>[2x]MNSKIRIGIVGYGNIGKGVEKAIKQNDDMELEAIFTRRDINKVDSNNSKLVHISRLELYKDTVDVMILCGGSATDLVEQGPMIAS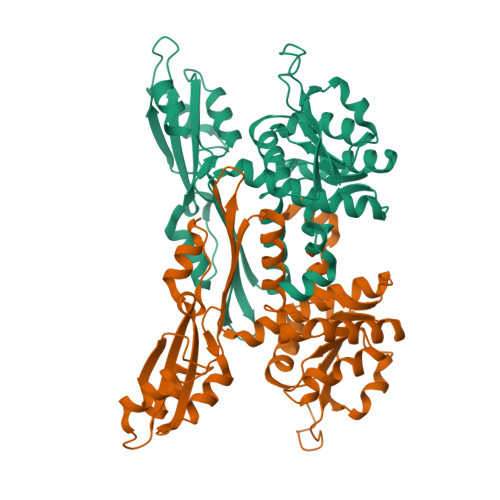QFNTVDSFDNHGRIPQHFERMDEISKKAGNISLISTGWDPGLFSLNRLLGESILPKGKTHTFWGKGVSLGHSDAIRRVQGVKNGIQYIIPIKGALDKARSGEQCDFTTREKHEMVCYVVPEENADLKKIEQDIKTMPDYFADYNTTVHFITEEELKLNHAGLSNGGFVIRSGNTQGGAKQVMEFNLNLESSAEFTSSVLVAYSRAIYKLSKEGKKGAVTVLDIPFSYLSPKTPEELRKELL>[12x]MSFEEVVQTLASLATVVQQQTIASESLEQRITSLENGLK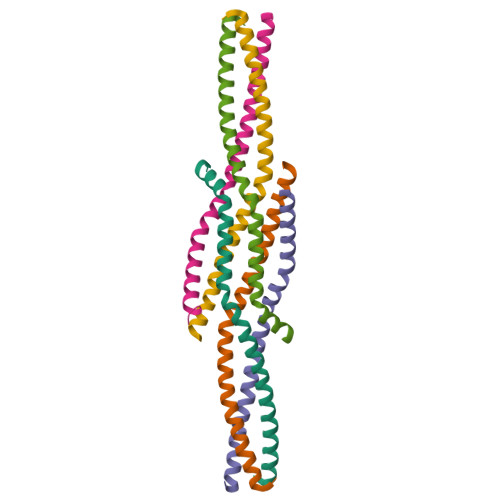PVYDMAKTISSLNRVCAEMVAKYDLLLEHHHHHH> TLHDKQIRVCHLFEQLSSATVIGDGDKHKHSDRLKNVGKLQPGAIFSCFHPDHLEEARHLYEVFWEAGDFNDFIEIAKEARTFVNEGLFAFAAEVAVLHRDDCKGLYVPPVQEIFPDKFIPSAAINEAFKKAHVRPEFDESPILVDVQDTGNILDPEYRLAYYREDVGINAHHWHWHLVYPSTWNPKYFGKKKDRKGELFYYMHQQMCARYDCERLSNGMHRMLPFNNFDEPLAGYAPHLTHVASGKYYSPRPDGLKLRDLGDIEISEMVRMRERILDSIHLGYVISEDGSHKTLDELHGTDILGALVESSYESVNHEYYGNLHNWGHVTMARIHDPDGRFHEEPGVMSDTSTSLRDPIFYNWHRFIDNIFHEYKNTLKPYDHDVLNFPDIQVQDVTLHARVDNVVHTFMREQELELKHGINPGNARSIKARYYHLDHEPFSYAVNVQNNSASDKHATVRIFLAPKYDELGNEIKADELRRTAIELDKFKTDLHPGKNTVVRHSLDSSVTLSHQPTFEDLLHGVGLNEHKSEYCSCGWPSHLLVPKGNIKGMEYHLFVMLTDWDKDKVDGSESVACVDAVSYCGARDHKYPDKKPMGFPFDRPIHTEHISDFLTNNMF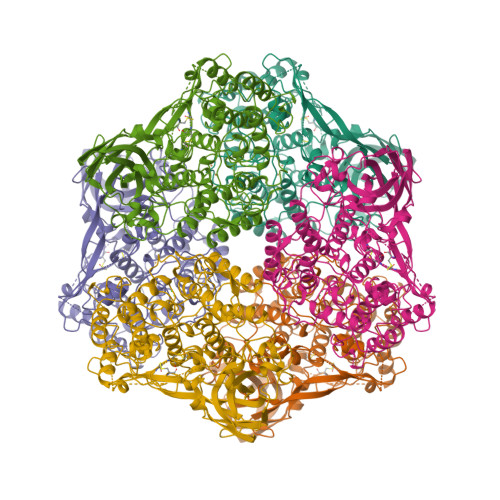IKDIKIKFHE Cellular respiration complexes convert redox energy into a transmembrane electrochemical proton gradient, which is used to synthesize adenosine triphosphate (ATP) or to transport various substances. In summary, we solved the 3.3 Å structure of respiratory complex III from the hyperthermophilic chemoautotrophic ϵ‐proteobacterium Aquifex aeolicus and revealed the structural basis for the hyperstability of proteins in an extreme thermal environment. The two cyt. b protomers bind to each other mainly through TMH1 and TMH4 to form a stable dimer. Several residues unique for thermophilic bacteria were detected that provide additional stabilization for ligand binding and for the structure of the whole complex.

1 complex from A. aeolicus has been shown to use a 1,4‐naphthoquinone (NQ), as a special substrate, to mediate electron transfer.9a In our cryo‐EM structure, several NQ molecules can be clearly traced in both the Qi site and on the cytoplasmic side, but none are around the Qo site. In particular, a well‐defined density map for a NQ is clearly visible in the Qi pocket formed by TMH1, TMH4 and TMH5 of the cyt. b. In the structure, we found density for two 1,4‐naphthoquinone substrates in the Qi site of cyt. b, around Arg222 residues on TMH4. The tail of the 1,4‐naphthoquinone stretches towards the membrane core outside of the binding pocket without interacting with cyt. b. Importantly, Arg222 residue is replaced by a histidine in R. sphaeroides and B. taurus. Compared with the short histidine residue, the positively charged side chain of Arg222 is closer to the oxygen atom of NQ. We find that a residue unique to the thermophiles, Tyr61 of cyt. b, is involved in this dimer interaction. The phenyl‐hydroxy of Tyr61 in TMH1 of one protomer binds to the nitrogen atom of Arg197 in TMH4 of another protomer enhancing the interactions between the two cyt. b protomers. In our structure, this WF‐rich TMH1 binds to the hydrophobic surface of the TMH region of the complex in the phospholipid layer. Importantly, this kind of interaction leads to the formation of a deep hydrophobic groove, which traps a phospholipid molecule.

>MEASRRDFISIGIGALGAVGGLGALYALVRVMLEPSEIAALGAKTEIDVSKIQPMQVRVTSWKGKTLFAIRLPKDFKPEGYTLKKGALNSKGTTNYEILKGHDVFALVGVCTHLGCIPLWKPQGEGGINKPVFHCPCHGGLYTPYGDVIGGPPPRPLFIPPQKLEGNKLIVGVEGFVKELI[2x];>[2x]MGLIEKIVDWIDERAHVREIYRTQMVEYKVAKNLTFPYVFGILALVTFAIQIISGMVLILYYKPSIADAFDSATYSIMGEIPFGWLFRHIHATGANFFMAIVYLHMFTGIYYNAYKRPRELVWIVGWLIYFVLILTALSGYLLPWGQLSYWGFIVTTEIPGSLADAPILKPIFKAIAETIVLWMKGGYVVTDVTLGRVFGSHVLIYPLILLALVGIHLYLVRAAGISNPEGIEYDKKKNPDKFVPFHPYMTLKEGAYVMWYLAVFFFFVFFHISHFLPPENFEPANPLKTPAHIAPEWYLLGYYEVFRSIPSKFWGFVAFNALLLLLLLLPFLDFSPLKSARRRPLFFVMFVIFMISSMALTILGTMPPTPQNAKLGLIFAALVFAFFISLPIISFIEYGWYKAKGGQQE;>[2x]MNTWGLIKTIFFAGSTLVFFFLLWFYNPFKHVEHYEVDEEVKAIIDNPWKKTESGKTIAEEGRELFIASCSSCHSLRYDGIYIMSVAANPKWKNIEKTSGRPVYRFGTLYKDRFFVPKDVYEAFAHDDIQGLKASLGQVPPDLSSMYLARGEGYLYQFILNPQKVLPGTTMPQLFNPQFDPQAKEKVAKIVAYMKSVNTPPPKESAKRTVMGVIVIAYFIVMGLLLWKYRENLLKRLGYH>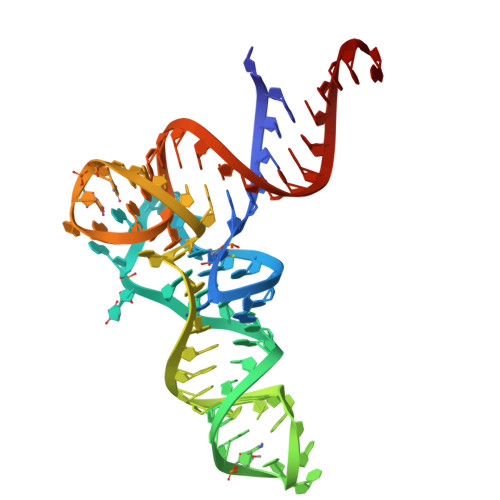 CGCGGGGUGGAGCAGCCUGGUAGCUCGUCGGGCUCAUAACCCGAAGAUCGUCGGUUCAAAUCCGGCCCCCGCAACCA> SMDAFEKVRTKLETQPQEEYEIINVEVKHGGFVYYQEGCCLVRSKDEEADNDNYEVLFNLEELKLDQPFIDCIRVAPDEKYVAAKIRTEDSEASTCVIIKLSDQPVMEASFPNVSSFEWVKDEEDEDVLFYTFQRNLRCHDVYRATFGDNKRNECFYTEKDPSYFVFLYLTKDSRFLTINIMNKTTSEVWLIDGLSPWDPPVLIQKRIHGVLYYVEHRDDELYILTNVGEPTEFKLMRTAADTPAIMNWDLFFTMKRNTKVIDLDMFKDHCVLFLKHSNLLYVNVIGLADDSVRSLKLPPWACGFIMDTNSDPKNCPFQLCSPIRPPKYYTYKFAEGKLFEETGHEDPITKTSRVLRLEAKSKDGKLVPMTVFHKTDSEDLQKKPLLVHVYGAYGMDLKMNFRPERRVLVDDGWILAYCHVRGGGELGLQWHADGRLTKKLNGLADLEACIKTLHGQGFSQPSLTTLTAFSAGGVLAGALCNSNPELVRAVTLEAPFLDVLNTMMDTTLPLTLEELEEWGNPSSDEKHKNYIKRYCPYQNIKPQHYPSIHITAYENDERVPLKGIVSYTEKLKEAIAEHAKDTGEGYQTPNIILDIQPGGNHVIEDSHKKITAQIKFLYEELGLDSTSVFEDLKKYLKF

Congenital myasthenic syndrome-22 (CMS22, OMIM 616224) is a rare genetic disorder caused by deleterious genetic variation in the prolyl endopeptidase-like (PREPL) gene. The PREPL protein consists of 2 structural domains: an amino-terminal 7-bladed β-propeller domain and a carboxy-terminal α/β-hydrolase fold catalytic domain connected by a hinge loop. The active site is comprised of the triad residues Ser559, Asp645, and His690. However, in contrast to its homologues PREP and OpdB, PREPL does not appear to possess protease activity despite the structural similarities.

To investigate the potential impact of the patient variants on PREPL conformation we solved the structure of p.Arg243Cys mutant using cryoelectron microscopy. This PREPL mutant was chosen due to its ability to be purified to higher concentrations compared with the other PREPL variants and its stable behavior on the cryo-EM grids. The resulting map was resolved at a resolution of 4.01 Å (using the FSC 0.143 criterion). Therefore, this structural study shows that the Arg243Cys variant did not affect the ternary structure of PREPL. Arg243 is positioned on PREPL in the loop connecting the β-11 and β-12 sheets of the third blade of the propeller and is not conserved across the homologous PREP, OpdB, and AAP. This residue resides in an exposed region on the protein surface, where neither the original arginine nor the cysteine undergoes any interactions with neighboring residues. Based on its location in the PREPL structure, it is not surprising that the variant retains catalytic activity but, instead, may affect protein-protein interactions mediated by the β-propeller. Moreover, we evaluated the cleavage of DIFMUO by CMS22 PREPL variants, where we saw that PREPL p.Arg243Cys (102.6 ± 26.2) had fully conserved catalytic activity, while PREPL p.Arg647Gln (43.8 ± 8.3) showed a 2-fold decrease in substrate cleavage activity compared with the WT (100.0 ± 23.6). We next assessed the folding and thermal stability of PREPL mutants by circular dichroism (CD) spectroscopy. p.Arg243Cys, p.Arg647Gln, and p.Ser559Ala PREPL share the same secondary structure as the WT protein. They all exhibited similar thermal stability, with the melting temperature (Tm) of PREPL WT and the p.Ser559Ala and p.Arg647Gln mutants calculated to be 63.5°C, while the melting temperature of p.Arg243Cys was 61.5°C. Their unfolding process displayed a 2-step pattern indicative of the presence of 2 domains as expected: the helical catalytic domain and the β-propeller comprised of β sheets. PREPL p.Arg243Cys had 7 decreased (NDUFV2, MRPL11, MRPS12, ARPC5L, DCTN5, DISC1, MDM1) and 1 increased interaction (UBL5); PREPL p.Ile412Arg had 8 decreased interactions (NDUFV2, MRPL11, MRPS12, STX5, ARPC5L, DCTN5, DISC1, MDM1); and PREPL p.Arg647Gln had 5 decreased (NDUFV2, MRPL11, STX5, ARPC5L, DCTN5) and 3 increased interactions (UBL5, ADM2, DISC1).> MSHHHHHHKNVPKGVLDKKNGREQRKTEQNVFNVDPASPWRHELLSFDECVSSALKYSTTPLQNTYKRIGNNQLNKNPSFAMFWDSMGRAMELYYSLRESPDFNAYRVSRLIHLLHNGLRSTRDQLVKLSRKPDYDSQSFHKE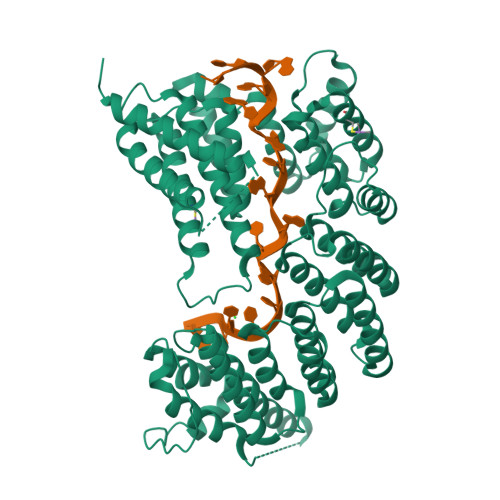MMNFLCNSLKDISDDILIGKVSVSGYGATHLLTSFKELSFDDDCIRIWEASKNLSDETTSQAFQEPKVVGFMLPLLYAKTRSLTEPNELYNQIIQSKEFIHPNLYSGLIKVFIKAEDYEKALSLFGQLCEKAEVRNYGYLIETHLSFIGDSKNLTLAESFFDKIINDEMPYKIILQVSTVNSFLQNIWKAQNDFDHVYRIWEKAVKFYGNTVNPGILSSLNNTFFTIFFENYINDNINGFRKLQEIITFYSGVKKIDEPFFNVMLTRASIWHERSIIDFIDKNYTLYHIPRTIISYRILLKSLGSIDNTNNEEILDRWLELVKKLNELGQQYIANADLSALRDATVVWSQSKRDEKVFSAKAKGTPATTTTTEDDIKVPKPLENLKNEDSTSNSEDRIELYLKILKRYTPYFRATKQVYRYTTGCAESYPILNEYLSGYSDLSAEDIPVPQLHSFIAKEQ> GSHMDYLVTEEEINLTRGPSGLGFNIVGGTDQQYVSNDSGIYVSRIKENGAAALDGRLQEGDKILSVNGQDLKNLLHQDAVDLFRNAGYAVSLRVQHRLQVQGSAYGSVKAYTNFDAERDALNIETAIKTKGVDEVTIVNILTNRSNEQRQDIAFAYQRRTKKELASALKSALSGHLETVILGLLKTPAQYDASELKASMKGLGTDEDSLIEIICSRTNQELQEINRVYKEMYKTDLEKDIISDTSGDFRKLMVALAKGRRAEDGSVIDYELI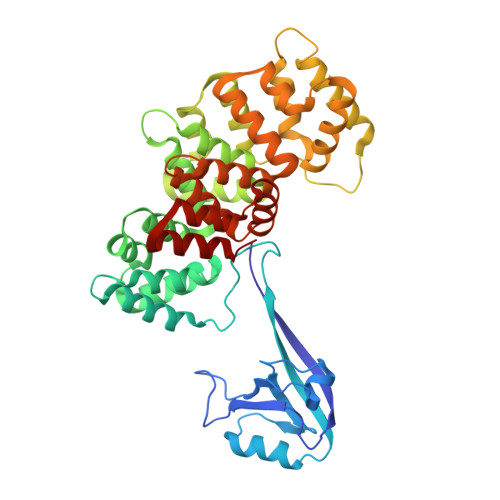DQDARDLYDAGVKRKGTDVPKWISIMTERSVPHLQKVFDRYKSYSPYDMLESIRKEVKGDLENAFLNLVQCIQNKPLYFADRLYDSMKGKGTRDKVLIRIMVSRSEVDMLKIRSEFKRKYGKSLYYYIQQDTKGDYQKALLYLCGGDD> MAQQRALPQSKETLLQSYNKRLKDDIKSIMDNFTEIIKTAKIEDETQVSRATQGEQDNYEMHVRAANIVRAGESLMKLVSDLKQFLILNDFPSVNEAIDQRNQQLRALQEECDRKLITLRDEVSIDLYELEEEY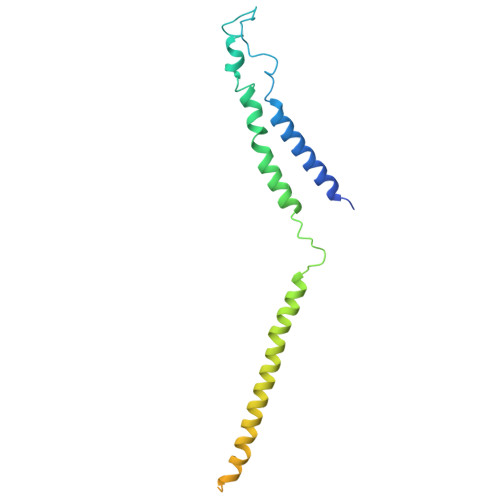YSSSSSLCEANDLPLCEAYWRLDLDADSADGLSAPLLASPETGAGPLQSAAPVHSHGGGPGPTEHT> ALWQFNGMIKCKIPSSEPLLDFNNYGCYCGLGGSGTPVDDLDRCCQTHDNCYKQAMKLDSCKVLVDNPYTNNYSYSCSNNEITCSSENNACEAFICNCDRNAAICFSKVPY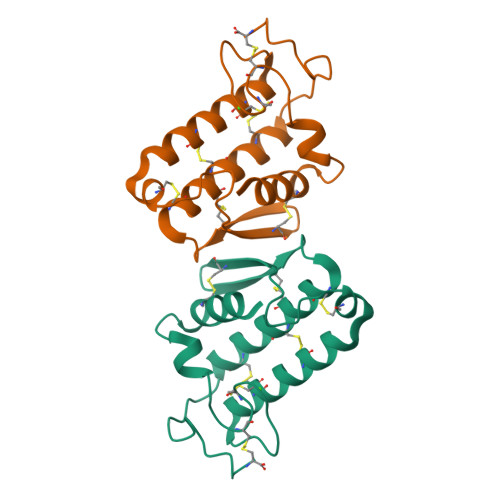NKEHKNLDKKNC> ASSVNELENWSKWMQPI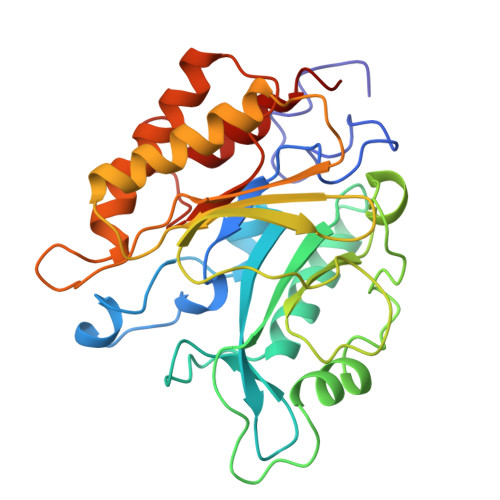PDSIPLARISIPGTHDSGTFKLQNPIKQVWGMTQEYDFRYQMDHGARIFDIRGRLTDDNTIVLHHGPLYLYVTLHEFINEAKQFLKDNPSETIIMSLKKEYEDMKGAEDSFSSTFEKKYFVDPIFLKTEGNIKLGDARGKIVLLKKYSGSNEPGGYNNFYWPDNETFTTTVNQNANVTVQDKYKVSYDEKVKSIKDTMDETMNNSEDLNHLYINFTSLSSGGTAWNSPYYYASYINPEIANYIKQKNPARVGWVIQDYINEKWSPLLYQEVIRANKSLIKE> DTKEQRILRYVQQNAKPGDPQSVLEAIDTYCTQKEWAMNVGDAKGQIMDAV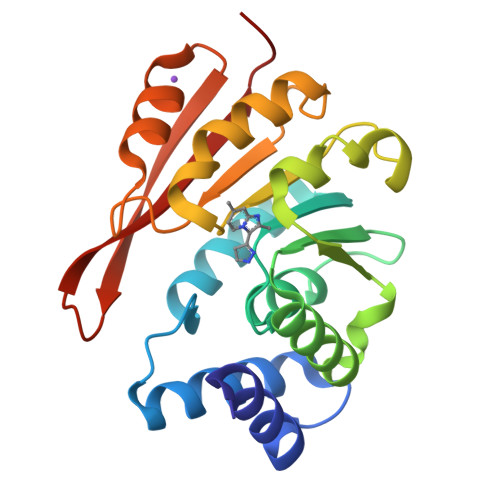IREYSPSLVLELGAYCGYSAVRMARLLQPGARLLTMEINPDCAAITQQMLNFAGLQDKVTILNGASQDLIPQLKKKYDVDTLDMVFLDHWKDRYLPDTLLLEKCGLLRKGTVLLADNVIVPGTPDFLAYVRGSSSFECTHYSSYLEYMKVVDGLEKAIYQGPS>MADDGSITAPEQGTLVGGVIAEPSAQMSAAADMATGKSVDSEWEAFFSFHTSVNWSTSETQGKILFKQALGPLLNPYLTHLAKLYVAWSGSIDVRFSISGSGVFGGKLAAIVVPPGVDPVQSTSMLQYPHVLFDARQVEPVVFTIPDLRSTLYHLMSDTDTTSLVIMIYNDLINPYANDANSSGCIVTVETKPGSDFKFHLLKPPGSMLTHGSVPSDLIPKSSSLWIGNRYWTDITDFVIRPFVFQANRHFDFNQETAGWSTPRFRPITVTISQKGGEKLGIGIATDFIVPGIPDGWPDTTIPSKLTPAGDYAV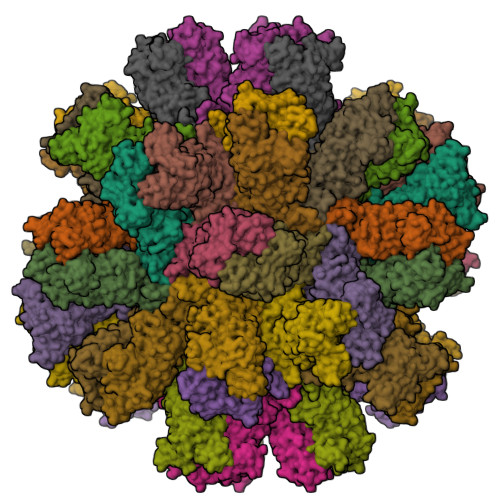TTSNGTDITTPREYDSANEIVNNTNFKSMYICGALQRAWGDKKISNTAFITTATVEGNNLEPSNVINPTKIAVFQDNHVNRDVQTSDVTLALLGYTGIGEEAIGADRDKVVRISVLPETGARGGNHPIFYKNTVKLGYVIRSIDVFNSQILHTSRQLSLNNYLLPPDSFAVYRIIDANGSWFDIGIDSDGFSFVGVSNIGKLEFPLSASYMGIQLAKIRLASNIRSTMTKL[20x]>MKSSHHHHHHENLYFQSNAKSPTDIGRNLARQWQRSSVRLERLLNPGSWPQSLNIGKPSARLFTDNIQAVLRHVENWRSVNVGKVDWEPVSYRAGLAPISLPMRWHLRSPSEWIAASDDPRVSQEYAQLEYLVEQVDSAFHTLLVAQRSLWLTRTPEEVVATAQLATQLAPGCAQGRPLRLLAEHGVDTKFFERNATLLTKLLDERFEGAASEQGLTTFLDAFEESSHWVLVVPLQPGLLPFKRLRLTTSELAETPLPGSRLLVVENEQCVHLLPETLPDTLAVLGAGLDLHWLASAHLAGKQIGYWGDMD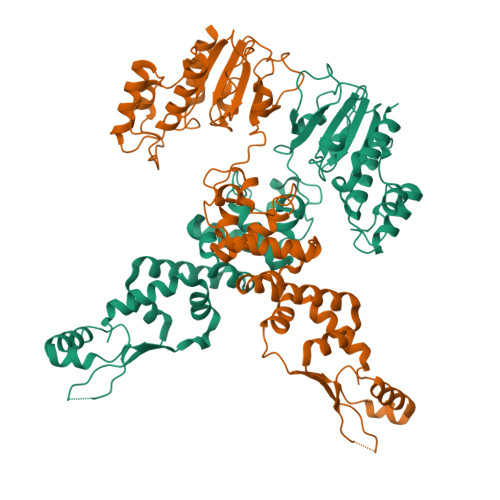TWGLLMLARARLHQPAVEALLMEQELFEQHSQGNTVVEPAKALESAPPGLLADEADFYRYLLVQERGRLEQEYLPKAQVELAIRKWAR[2x]> MAAVVKSVALAGRPTTPDRVHEVLGRSMLVDGLDIVLDLTRSGGSYLVDAITGRRYLDMFTFVASSALGMNPPALVDDREFHAELMQAALNKPSNSDVYSVAMARFVETFARVLGDPALPHLFFVEGGALAVENALKAAFDWKSRHNQAHGIDPALGTQVLHLRGAFHGRSGYTLSLTNTKPTITARFPKFDWPRIDAPYMRPGLDEPAMAALEAEALRQARAAFETRPHDIACFVAEPIQGEGGDRHFRPEFFAAMRE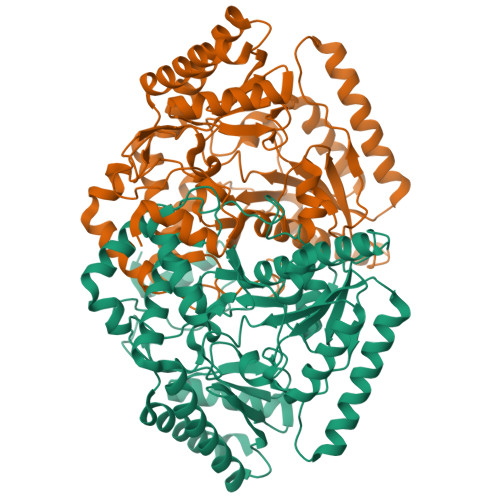LCDEFDALLIFDEVQTGCGLTGTAWAYQQLDVAPDIVAFGKKTQVCGVMAGRRVDEVADNVFAVPSRLASTWGGNLTDMVRARRILEVIEAEGLFERAVQHGKYLRARLDELAADFPAVVLDPRGRGLMCAFSLPTTADRDELIRQLWQRAVIVLPAGADTVRFRPPLTVSTAEIDAAIAAVRSALPVVT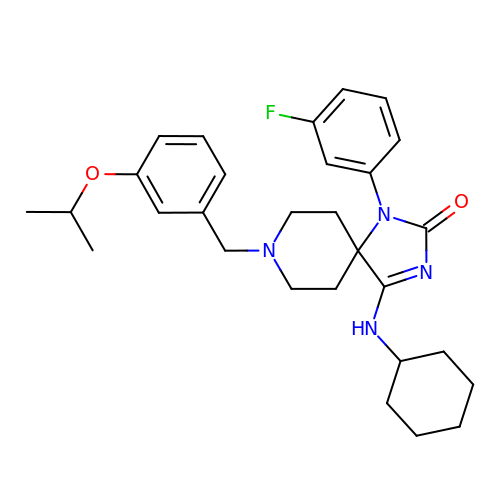4-(cyclohexylamino)-1-(3-fluorophenyl)-8-[3-(propan-2-yloxy)benzyl]-1,3,8-triazaspiro[4.5]dec-3-en-2-one | C29 H37 F N4 O2 | KZMSAJWZLCSCQP-UHFFFAOYSA-N> GPGSKDFQGMLEYKREDEQKLVKNLILELKPRGVAVNLIPGLPAYILFMCVRHADYLNDDQKVRSLLTSTINSIKKVLKKRGDDFETVS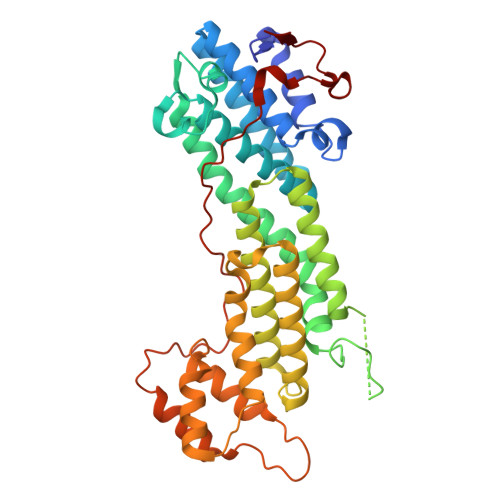FWLSNTCRFLHCLKQYSGEEGFMKHNTSRQNEHCLTNFDLAEYRQVLSDLAIQIYQQLVRVLENILQPMIVSGMLEHETIQGVSGVKPTGLRKRTSSIADEGTYTLDSILRQLNSFHSVMCQHGMDPELIKQVVKQMFYIVGAITLNNLLLRKDMCSWSKGMQIRYNVSQLEEWLRDKNLMNSGAKETLEPLIQAAQLLQVKKKTDDDAEAICSMCNALTTAQIVKVLNLYTPVNEFEERVSVSFIRTIQMRLRDRKDSPQLLMDAKHIFPVTFPFNPSSLALETIQIPASLGLGFIARV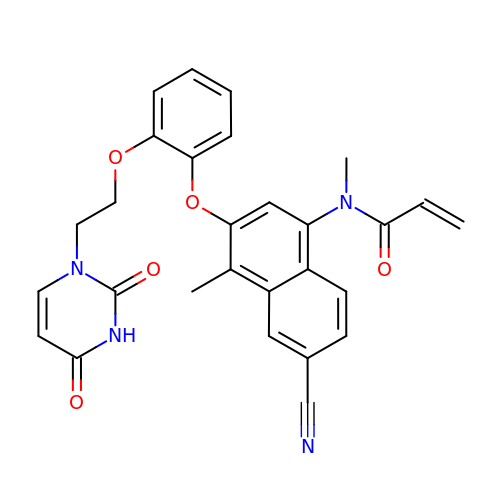N-(6-cyano-3-{2-[2-(2,4-dioxo-3,4-dihydropyrimidin-1(2H)-yl)ethoxy]phenoxy}-4-methylnaphthalen-1-yl)-N-methylprop-2-enamide | C28 H24 N4 O5 | OFTCTICPJPOVAI-UHFFFAOYSA-N> MRINSELANKFSASTVHLEHITTALSCLTPFGSKDDVLIFIDADGLSFVRENNHVIKIQLLLSRELFMSYSYRNETEDHMKLCVKINHILDSVSVMNRNSDDIVECTLSYDGHGSPFVLIFEDSFISERVEYSTYLIKDFDTNGLELDRERISFEAIIKGEALHSALKDLKEIGCKECYVYAKTEANDENVFAL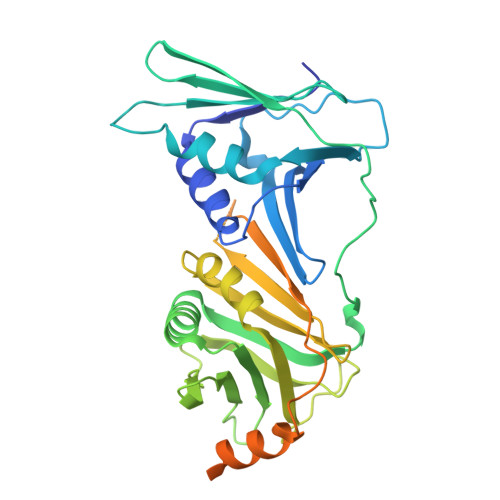ISKSQLGFSKIKLPSNRSILEKLQVFDGDSTTVIDGFAVIGFFDFTSFDKIRKSTKIASKVLFRMDVHGVLSVNILSQTDDVIITDTTRPSNNRPGSIRQLQLPKDYPGIVIEVCMLEKESIDEAAQTEIELLMETNELGNRNSFKKSTIRKRYGTDKGNETSNDNLLQLNGKKIKLPSEEENNKNRESEDEENHCKYPTKDIPIFF> G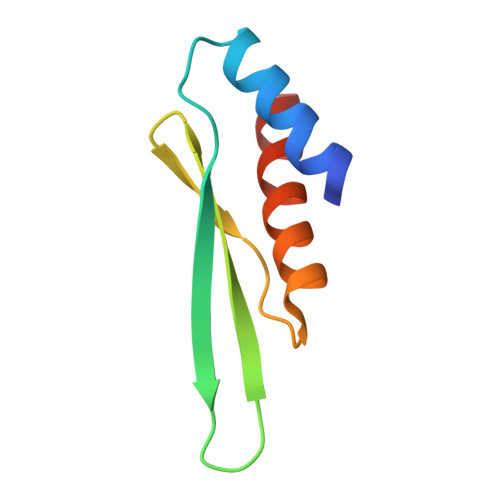SHGLCKNLLQEYAQKMNYAIPLYQCQKVETLGRVTQFTCTVEIGGIKYTGAATRTKKDAEISAGRTALLAIQSDT>[2x]HMTTAQHPTDEDLLARVLVPYKDHCKYLRSAVVTESDTGRAVARCEFAIPESCYIDDTGHLNSVEVNICYNQMMYYLVAKSVKEGLLA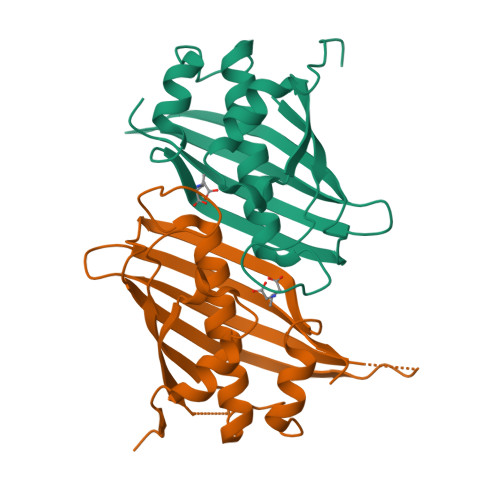GFESWTLDDFWKHQLPDILIARFASNFRRPVNPRAFSGEMEFQSVTRRAPAGGIPFLHAETAYRYWDADSGRCDGEAVLAFVNIP> XKKLLKCLK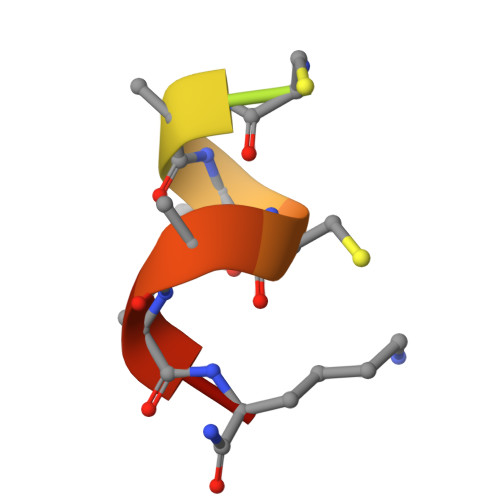CLLKX> GSSGSSGMQIGKIIKVSGPLVMAENMSEASIQDMCLVGDLGVIGEIIEMRQDVASIQVYEETSGIGPGEPVRSTGEALSVELGPGIISQMFDGIQRPLDTFMEVTQS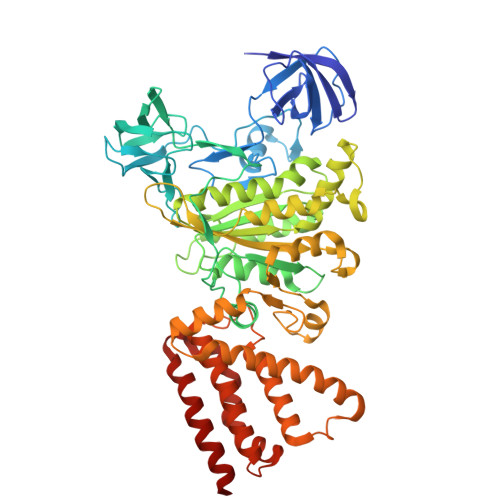NFLGRGVQLPALDHEKQWWFEATIEEGTEVSAGDIIGYVDETKIIQHKIMVPNGIKGTVQKIESGSFTIDDPICVIETEQGLKELTMMQKWPVRRGRPIKQKLNPDVPMITGQRVIDTFFPVTKGGAAAVPGPFGAGKTVVQHQIAKWSDVDLVVYVGCGERGNEMTDVVNEFPELIDPNTGESLMERTVLIANTSNMPVAAREASIYTGITIAEYFRDMGYDVAIMADSTSRWAEALREMSGRLEEMPGDEGYPAYLGSRLAEYYERSGRVIALGSDQREGSITAISAVSPSGGDISEPVTQNTLRVVKVFWGLDSSLAQKRHFPSINWIQSYSLYSTEVGRYMDQILQQDWSDMVTEGMRILQEEEQLNEIVRLVGIDSLSDNDRLTLEVAKSIREDYLQQNAFDDVDTFTSREKQFNMLKVILTFGKEARKALSLGAYFNEIMEGTVAVRERISRSKYIPEEELAKISSINEEIKETIQLIVSE Cys-ketimine 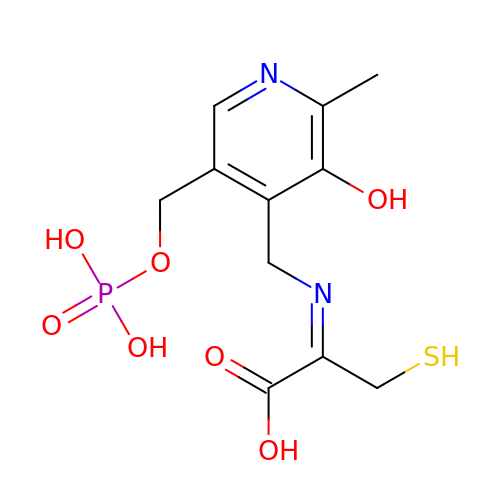| C11 H15 N2 O7 P S | KPYIACOPTFGBII-UKTHLTGXSA-N>SNAMTAVNYPFVDTMDKFDKITKGLIFEHQAEGESETMISHELSILDNDGVVHSLHFSQITSLIDTITGKHPSLELPPQLFLITQYLLEDLKEVGEKGFVITEYFIDVLPTGNKAIFRGTLAHKSTVDGHPDFDPSSTISKKEFEFSLNQFSILQQIALSHCIANLHEECAGFRGTFDVEYTFHWTPFAFNVKFSE[4x]

The phage nuclear shell is composed primarily of one protein, termed chimallin (ChmA) or phage nuclear enclosure (PhuN), which forms a single-layer-thick flexible lattice that separates the phage genome from the bacterial cytoplasm. Pores in the ChmA lattice are less than ~2 nm in width, large enough to pass metabolites but too small for passage of most proteins or messenger RNAs (mRNAs). We found that one of these proteins (gp2) associated directly with self-assembled ChmA in vitro, suggesting that it is an integral phage nuclear shell protein and prompting us to name it ChmB. We identified a key protein, ChmB, at the center of this network that is likely to have multiple roles both as a pore for macromolecular translocation through the nuclear shell and for capsid docking and genomic DNA packaging.

To determine the structural basis for ChmB interactions with other proteins, we recombinantly purified the protein from several jumbo phages and determined a 2.6 Å resolution crystal structure of ChmB from the related phage PA1C (gp2; 38% identical to ΦPA3 gp2). ChmB formed a homodimer in solution, and the structure revealed an intertwined dimeric structure with the N terminus of each protomer forming a short β-strand and an α-helix that pack against the C-terminal globular domain of its dimer mate. Overall, the ChmB dimer adopts a distinctive U shape with dimensions of ~5 × 8 nm. NTS-mediated interactions define ChmA homotetramers that measure ~11.5 × 11.5 nm, whereas CTS-mediated interactions mediate interactions between neighboring tetramers. The distinctive U shape and overall dimensions of the ChmB dimer, at ~5 × 8 nm, suggest a model in which multiple ChmB dimers could line a hole created by the removal of four or more neighboring ChmA protomers from the lattice (two possibilities shown in Fig. 5b). Indeed, size-exclusion chromatography of ChmB at high concentration suggests a propensity for higher-order self-assembly that may be reinforced by integration into the ChmA lattice. Combined with our data showing that gp2 interacts directly with self-assembled ChmA, these data suggest that gp2 is an integral component of the phage nuclear shell that is directly involved in the docking and filling of capsids through an interaction with the portal. Based on these data, we propose that ChmB mediates capsid docking and genome packaging at the nuclear shell through a direct interaction with the portal protein. We next aligned ChmB homologs from jumbo phages that infect Pseudomonas species and identified two highly conserved surface residues: Q53 and A159 (ΦPA3 gp2 numbering). We generated point mutations of these residues (Q53A and A159D, respectively) designed to alter the ChmB surface and potentially disrupt specific protein–protein interactions.> SMPKLPENYTDETWQKLKEAVEAIQNSTSIKYNLEELYQAVENLCSYKISANLYKQLRQICEDHIKAQIHQFREDSLDSVLFLKKIDRCWQNHCRQMIMIRSIFLFLDRTYVLQNSMLPSIWDMGLELFRAHIISDQKVQNKTIDGILLLIERERNGEAIDRSLLRSLLSMLSDLQIYQDSFEQRFLEETNRLYAAEGQKLMQEREVPEYLHHVNKRLEEEADRLITYLDQTTQKSLIATVEKQLLGEHLTAILQKGLNNLLDENRIQDLSLLYQLFSRVRGGVQVLLQQWIEYIKAFGSTIVINPEKDKTM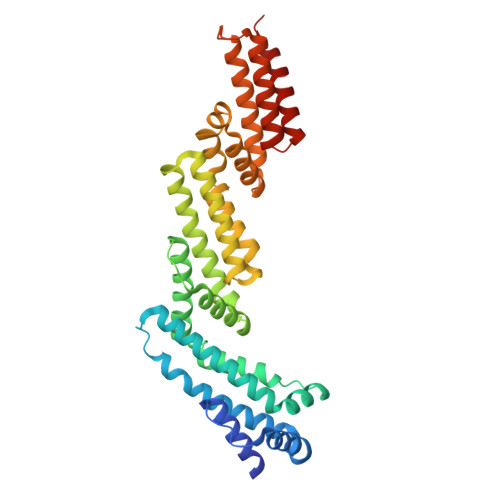RQELDDFKDKVDHIIDICFLKNEKFINAMKEAFETFINKRPN>[3x]GAMALEARLEQASILKKVVDAIKDLVQDCNFDCNDSGIALQAMDNSHVALVSMMLKAEGFSPYRCDRNIALGVNLTSLTKVLRAAQNEDILTLKAED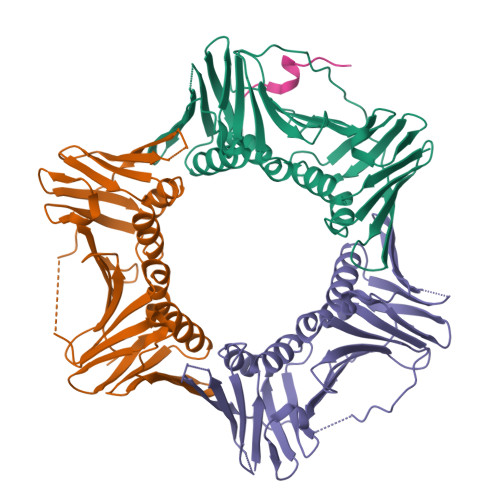APDVLNLVFESSETDRISEYDLKLMDIDQEHLGIPETEYAATITMPSNEFKRITTDLMAMSESVTIEANKDGVKFSCQGDIGNGSVTLRQHTNVEKPNESIEIELSEPVSLTFSLKYLVNFCKASALSNTVKICLSNEVPLLVEYSLGGSSYLRFYLAPKIGDDE;> GKGGQGSIMSWFAKK(1R,2R,4S,5R)-2-(benzo[b]thiophen-5-yl)methyl-1,4,5-trihydroxy-3-oxocyclohexane-1-carboxylic acid | 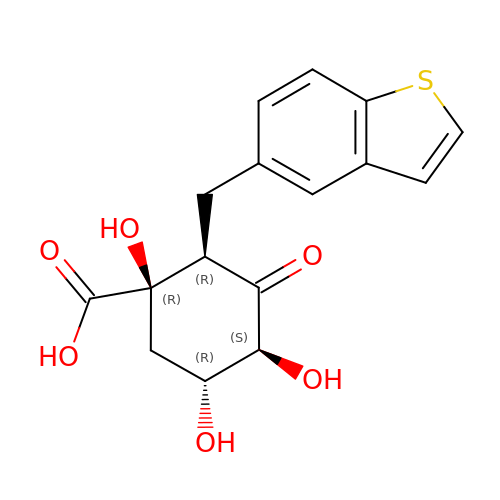C16 H16 O6 S | WFQJMZIPFQUOBR-FJXFWJLJSA-N> MAAACAVRGFTTARPMLTPNKVKVPGRKPQDEEDLTWAEADRKLTPEERYARDK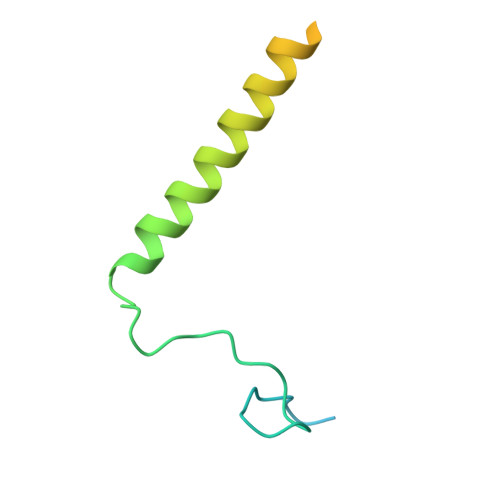QMALLDKMTSQVEELEKSHTEQKKSNKGVKAQIEAISRQLEALKAQLKE> MHHHHHHMVDEILKLKKEKGYIILAHNYQIPELQDIADFVGDSLQLARKAMELSEKKILFLGVDFMAELVKILNPDKKVIVPDRSATCPMANRLTPEIIREYREKFPDAPVVLFVNSTSE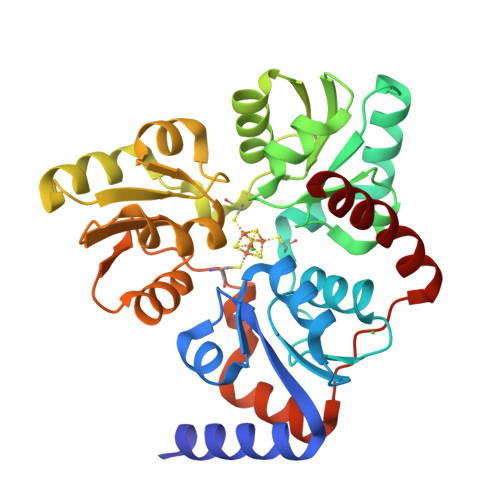CKTLADVICTSANAVEVVKKLDSSVVIFGPDRNLGEYVAEKTGKKVITIPENGHCPVHQFNAESIDAVRKKYPDAKVIVHPECPKPVRDKADYVGSTGQMEKIPERDPSRIFVIGTEIGMIHKLKKKFPDREFVPLEMAVCVNMKKNTLENTLHALQTESFEVILPKEVIEKAKKPILRMFELMG4S/3694 | C21 H20 N6 O2 | 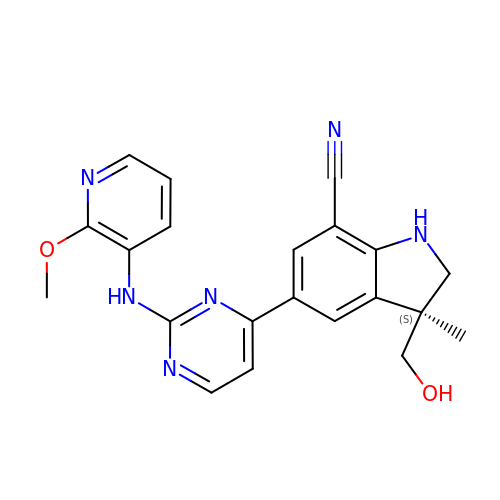PTVSCHCHSJTBBB-NRFANRHFSA-N> MYRAAASSFRRHLKGHGSKLGSTRSSTSAAVAARTSKGGLFSWLTGERSSSLPSLDIPLGGVVLPDPLPDSVEQSKTKITTLSNGLKIASETSPN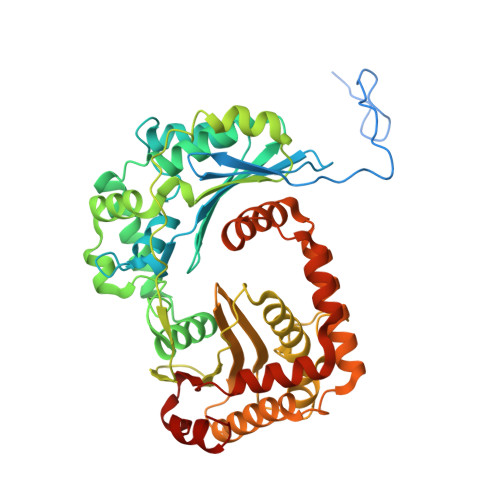PAASIGLYLDCGSIYETPFSSGASHLLERMAFKSTTNRSHFRIVREVEAIGGNIGASASREQMGYTFDALKTYVPQMVELLVDCVRNPAFLDWEVNEELRKVKAELGELSNNPQGLLLEAIHSAGYSGALAYPLLAPEAALNRLDGPSLEEFVAENYTAPRMVLAAAGVEHEELVSIAEPLLSDLPNVPRPDEPKSVYVGGDFRRHGESGGTHVALAFEVPGGWHKEKDAIVLTVLQMLMGGGGSFSAGGPGKGMHSRLYLRVLNEYQQIQSFSAFNSIFNNTGLFGIYASTSPDFAPKAVDIAAKELIAIASPGQVTQVQLDRAKKSTKSAVLMNLESRMIASEDIGRQILTYGERKPLEQFLKAVDEITLNDITKISQKIISSPLTMASYGDVLSVPSYESVNRKFHAK> GSLRELKVCLLGDTGVGKSSIVWRFVEDSFDPNINPTIGASFMTKTVQYQNELHKFLIWDTAGQERFRALAPMYYRGSAAAIIVYDITKEETFSTLKNWVRELRQHGPPSIVV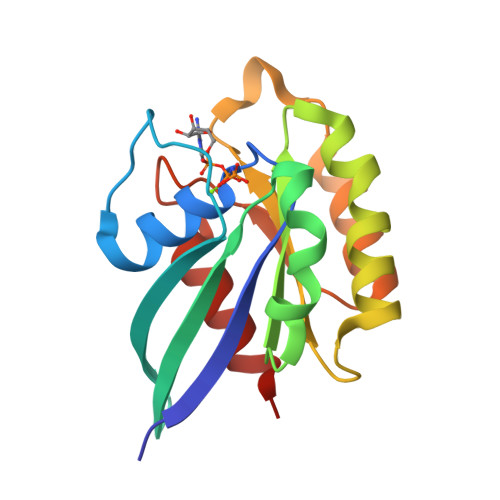AIAGNKCDLTDVREVMERDAKDYADSIHAIFVETSAKNAININELFIEISRRIPST> GKAFDDGVFTGIREINLSYNK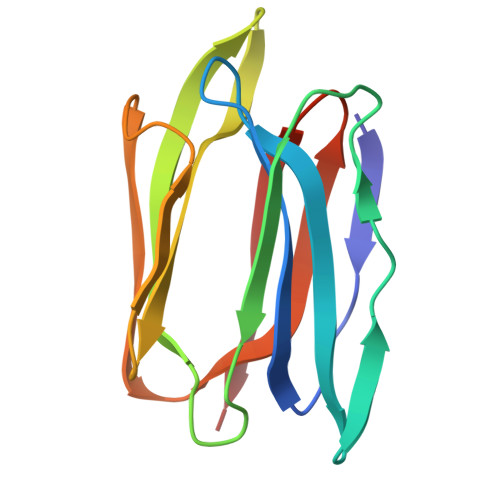ETAIGDFQVVYDLNGSPYVGENHKSFITGFTPVKISLDFPSEYIMEVSGYTGKVSGYVVVRSLTFKTNKKTYGPYGVTSGTPFSLPIENGLIVGFKGSIGYWLDYFSMYLSL>SNAMYDIYGEAALPADVRERLRITRDLAQAFHERAPEHDRAGDFPFENIEDLKASGYVRWTVPVEYGGLGLSLEEMLMHQEVLAKGDGSTALAIGWHVGILLHLRETGAFPDELFRMVCESVVKEGALINSCATEPATGSPSRGGKPETTAVKVPGGYRITGRKTFSTLSPALTWIMVTATVADEDVVGQFLVRKEDVEIVETWDTLGMRATGSHDIVLKDVFVPEERVIVIQRPGVQAERRPDGSGWLLHIPACYLGIALAARDFALEYAATYRPNTLPHPIAEVPHVEQKLGEMELKLLAARTLLYDLARRFDAASPEERVKLQPQFGAVKTLATN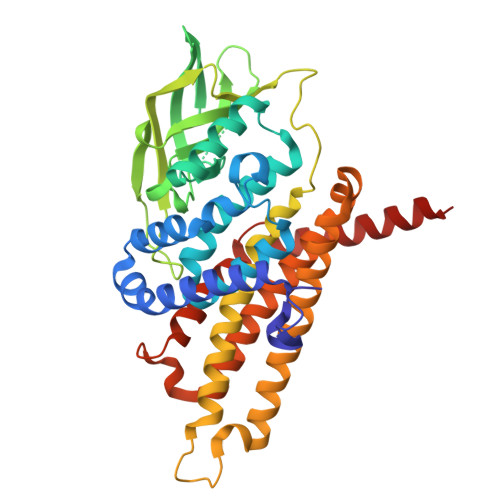AANQVVDLAMRVVGGRSLSRALPLERYYRDVRAGLHNPPMDDVVYRNLAKAALARRAAGQ[2x]>MATSASSHLNKGIKQMYMNLPQGEKIQLMYIWVDGTGEGLRCKTRTLDCDPKCVEELPEWNFDGSSTFQSEGSNSDMYLHPVAMFRDPFRRDPNKLVFCEVFKYNRKPAETNLRHSCKRIMDMVSSQHPWFGMEQEYTLMGTDGHPFGWPSNGFPGPQGPYYCGVGADKAYGRDIVEAHYRACLYAGIKITGTNAEVMPAQWEFQ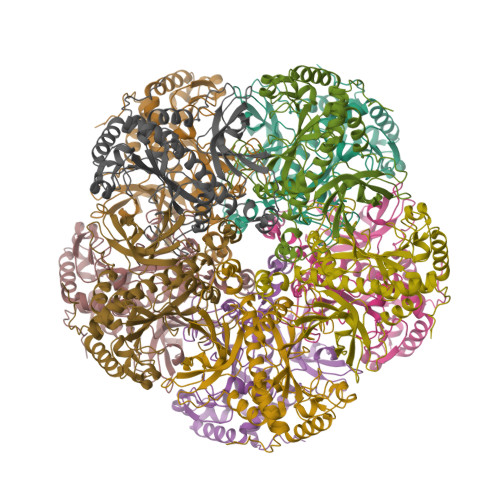IGPCEGIRMGDHLWVARFILHRVCEDFGVIATFDPKPIPGNWNGAGCHTNFSTKAMREENGLRCIEEAIDKLSKRHQYHIRAYDPKGGLDNARRLTGFHETSNINDFSAGVANRSASIRIPRIVGQEKKGYFEDRRPSANCDPYAVTEAIVRTCLLNETGDEPFQYK[10x]>[2x]MGSSHHHHHHSSGLVPRGSEIKFLKKEDVQNIDLNGMSKKERYEIWRRIPKVELHCHLDLTF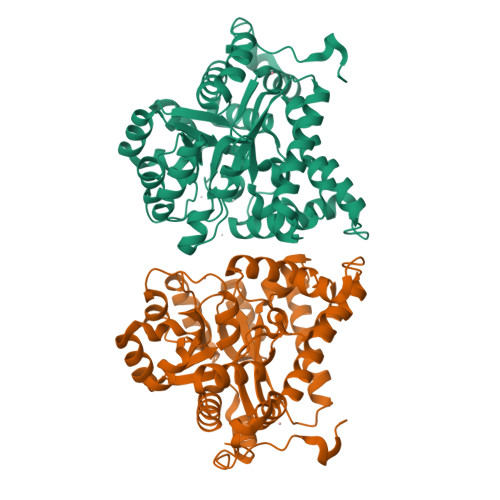SAEFFLKWARKYNLQPNMSDDEILDHYLFTKEGKSLAEFIRKAISVSDLYRDYDFIEDLAKWAVIEKYKEGVVLMEFRYSPTFVSSSYGLDVELIHKAFIKGIKNATELLNNKIHVALICISDTGHAAASIKHSGDFAIKHKHDFVGFDHGGREIDLKDHKDVYHSVRDHGLHLTVHAGEDATLPNLNTLYTAINILNVERIGHGIRVSESDELIELVKKKDILLEVCPISNLLLNNVKSMDTHPIRKLYDAGVKVSVNSDDPGMFLSNINDNYEKLYIHLNFTLEEFMIMNNWAFEKSFVSDDVKSELKALYF> MASMTGGQQMGRGSMSTKAIYPGTFDPITNGHIDIITRAASMFDRVILAIAASPSKKPMFDLEERVALATTALQHLPNVEVMGFSDLMANFARAQQANILIRGLRAVADFEYEMQLAHMNRHLMPELESVFL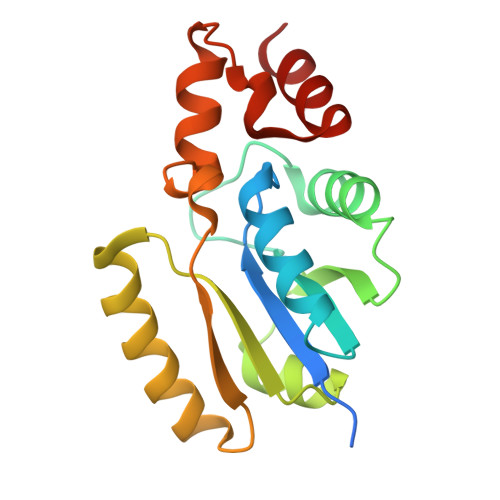MPSKEWSFISSSLVKEVARHAGDVTHFLPANVHQALMEKLK The extracellular calcium-sensing receptor (CaSR) is responsible for the maintenance of a stable blood Ca2+ level. CaSR is a class C G-protein-coupled receptor (GPCR). Ligand binding to CaSR takes place within a large extracellular Venus Flytrap (VFT) module that consists of two domains (LB1 and LB2). In addition, CaSR contains a cysteine-rich (CR) domain that connects the VFT module to the transmembrane region.

In the form II crystal structure, both protomers of CaSR ECD have the closed conformation associated with agonist binding (closed-closed). Surprisingly, the ligand-binding cleft of each protomer is solely occupied by an L-Trp molecule. Ca2+ is bound at four novel sites in the CaSR ECD structure, including one at the homodimer interface. Each CaSR ECD molecule also contains two PO43- ions. L-Trp facilitates extracellular domain closure of CaSR by contacting both LB1 and LB2 domains of the VFT module. The interactions between CaSR ECD and L-Trp are primarily mediated by hydrogen bonds. Third, the CR domains of the two subunits interact to form a large homodimer interface that is unique to the active state. Finally, the structural reorganization of CR domains reduces the distance between the C-termini of the two subunits from 83 Å to 23 Å. Site 4 is part of the homodimer interface formed upon agonist binding, bridging the LB2 domain of one subunit and CR domain of the second subunit. Our structural data indicate that the Ca2+ ion at site 4 stabilizes the active conformation of the receptor by facilitating homodimer interactions between the membrane-proximal LB2 and CR domains.

>[2x]MAFYSCCWVLLALTWHTSAYGPDQRAQKKGDIILGGLFPIHFGVAAKDQDLKSRPESVECIRYNFRGFRWLQAMIFAIEEINSSPALLPNLTLGYRIFDTCNTVSKALEATLSFVAQNKIDSLNLDEFCNCSEHIPSTIAVVGATGSGVSTAVANLLGLFYIPQVSYASSSRLLSNKNQFKSFLRTIPNDEHQATAMADIIEYFRWNWVGTIAADDDYGRPGIEKFREEAEERDICIDFSELISQYSDEEEIQHVVEVIQNSTAKVIVVFSSGPDLEPLIKEIVRRNITGKIWLASEAWASSSLIAMPQYFHVVGGTIGFALKAGQIPGFREFLKKVHPRKSVHNGFAKEFWEETFNCHLQEGAKGPLPVDTFLRGHEESGDRFSQSSTAFRPLCTGDENINSVETPYIDYTHLRISYNVYLAVYSIAHALQDIYTCLPGRGLFTNGSCADIKKVEAWQVLKHLRHLQFTNNMGEQVTFDECGDLVGNYSIINWHLSPEDGSIVFKEVGYYNVYAKKGERLFINEEKILWSGFSREVPFSNCSRDCLAGTRKGIIEGEPTCCFECVECPDGEYSDETDASACNKCPDDFWSNENHTSCIAKEIEFLSDYKDDDDK> MAANKPKGQNSLALHKVIMVGSGGVGKSALTLQFMYDEFVEDYEPTKADSYRKKVVLDGEEVQIDILD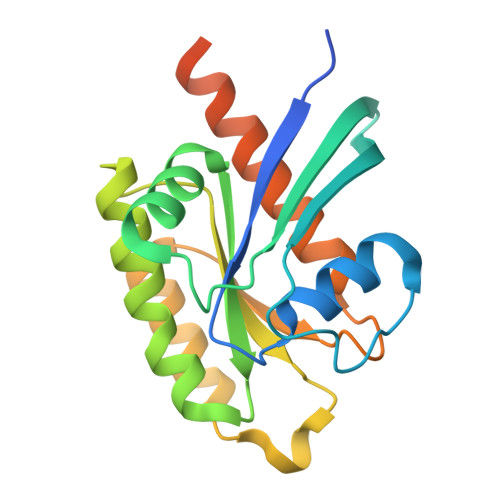TAGQEDYAAIRDNYFRSGEGFLCVFSITEMESFAATADFREQILRVKEDENVPFLLVGNKSDLEDKRQVSVEEAKNRAEQWNVNYVETSAKTRANVDKVFFDLMREIRARKMEDSKEKNGKKKRKSLAKRIRERCCIL> GTSLTRKQCDFTKLIMAGYDLELNNGSTQDFDVMFHGPNGTAYEGGIWKVHVTLPDDYPFASPSIGFMNKLLHPNVDEASGSVCLDVINQTWTPLYSLVNVFEVFLPQLLTYPN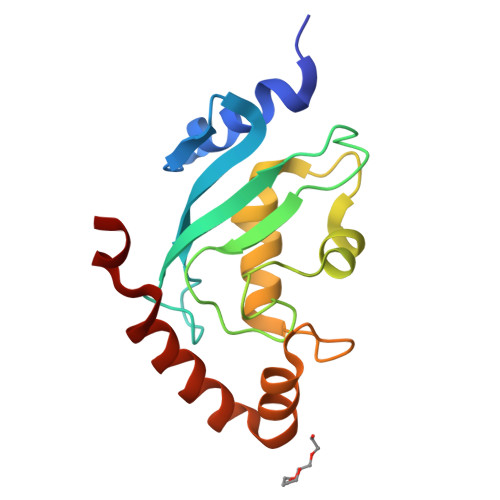PSDPLNSDAASLLMKDKNIYEEKVKEYVKLYASKDLWE>[4x]MMENIMKKRLLSTSISTLLLGLSVMPAFADEDVTAWRLFIADHDKPVVNVIDALDGDKLATFNVKGPANLSRSESGATIFAIQGSAGVVSTIASGIAFHDHGDHADIDIDAPKLLPLELTGKKPGHFVERQGKIAQWFDGEDSAQILGESAVLKGQKNITKVNVVAPHHGVAVPYDNYAVVSIPNPDDASKRPVGARVVDLQGKKVGDDALCPGLHGSAGSGDTFALSCETGLLL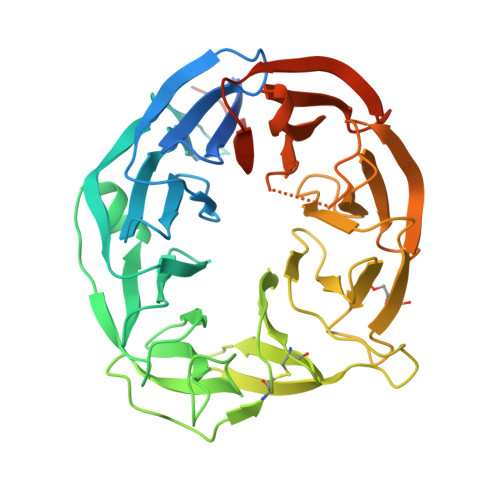ITQKNAAPVIRHLPYAKTLPEGSTSTLIGGKGMQYFIGNYGPDRIILVDPTESDSFRLIQLPTRRVHFVVDPVRAKFAYVFTEDGKLNQIDVLKGEISQSVRVTDPYSMDGHWNDPRPRIAVADNKIYVTDPLKSKIIVLDATSFKKTSEISVEGQPFNIVAVGGSGKVHGEHHDHEAHHHDDHAH> GVALGATRVIYPAGQKQEQLAVTNNDENSTYLIQSWVENADGVKDGRFIVTPPLFAMKGKKENTLRILDATNNQLPQDRESLFWMNVKAIPSMDKSKLTENTLQLAIISRIKLYYRPAKLALPPDQAAEKLRFRRSANSLTLINPTPYYLTVTELNAGTRVLENA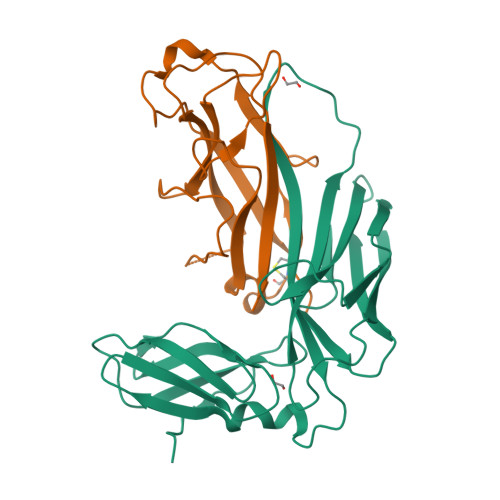LVPPMGESTVKLPSDAGSNITYRTINDYGALTPKMTGVMEHHHHHH;> AETCRIEAGDKQMTVNMGQISSNRFHAVGEDSAPVPFVIHLRECSTVVSERVGVAFHGVADGKNPDVLSVGEGPGIATNIGVALFDDEGNLVPINRPPANWKRLYSGSTSLHFIAKYRATGRRVTGGIANAQAWFSLTYQ(3R)-1-(3-hydroxy-9,10-dioxo-9,10-dihydroanthracene-2-sulfonyl)piperidine-3-carboxylic 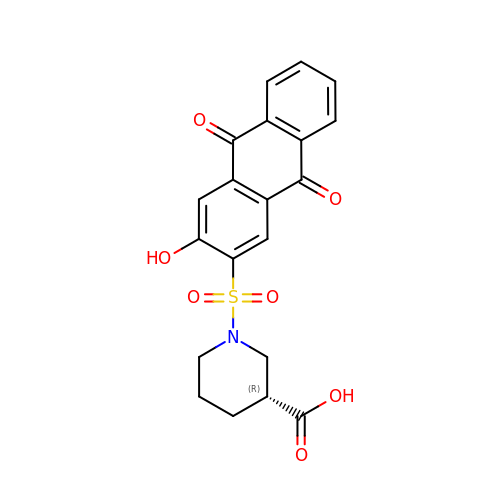acid | C20 H17 N O7 S | WJGDJAJWMMMYSV-LLVKDONJSA-N> QDSKYQCVKLNDGHFMPVLGFGTYAPAEVPKSKALEATKLAIEAGFRHIDSAHLYNNEEQVGLAIRSK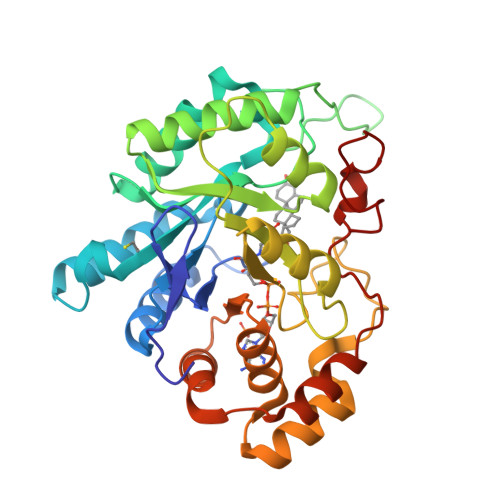IADGSVKREDIFYTSKLWCNSHRPELVRPALERSLKNLQLDYVDLYLIHFPVSVKPGEEVIPKDENGKILFDTVDLCATWEAVEKCKDAGLAKSIGVSNFNRRQLEMILNKPGLKYKPVCNQVECHPYFNQRKLLDFCKSKDIVLVAYSALGSHREEPWVDPNSPVLLEDPVLCALAKKHKRTPALIALRYQLQRGVVVLAKSYNEQRIRQNVQVFEFQLTSEEMKAIDGLNRNVRYLTLDIFAGPPNYPFSDEY>STAGKVIKCKAAVLWEEKKPFSIEEVEVAPPKAHEVRIKMVATGICRSDDHVVSGTLVTPLPVIAGHEAAGIVESIGEGVTTVRPGDKVIPLWTPQCGKCRVCKHPEGNFCLKNDLSMPRGTMQDGTSRFTCRGKPIHHFLGTSTFSQYTVVDEISVAKIDAASPLEKVCLIGCGFSTGYGSAVKVAKVTQGSTCAVFGLGGAGLSVIMGCKAAGAARIIGVDINKDKFAKAKEVGATECVNPQDYKKPIQEVLTEMSNGGVDFSFEVIGRLDTMVTALSCCQEAYGVSVIVGVPPDSQNLSMNPMLLLSGRTWKGAI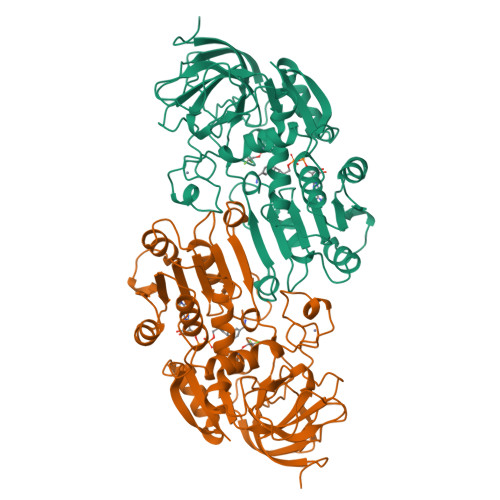FGGFKSKDSVPKLVADFMAKKFALDPLITHVLPFEKINEGFDLLRSGESIRTILTF[2x]>[2x]MSMAMSQSNRELVVDFLSYKLSQKGYSWSQFSDVEENRTEAPEGTESEAVKQALREAGDEFELRYRRAFSDLTSQL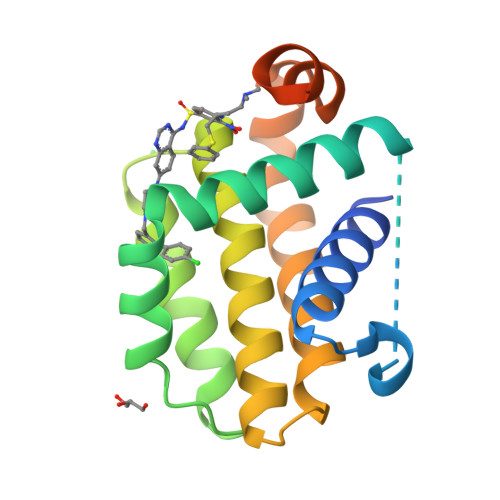HITPGTAYQSFEQVVNELFRDGVNWGRIVAFFSFGGALCVESVDKEMQVLVSRIAAWMATYLNDHLEPWIQENGGWDTFVELYGNNAAAESRKGQERLEHHHHHH>MNDPNLFVALYDFVASGDNTLSITKGEKLRVLGYNHNGEWCEAQTKNGQGWVPSNYITPVNS[2x];>APTMPP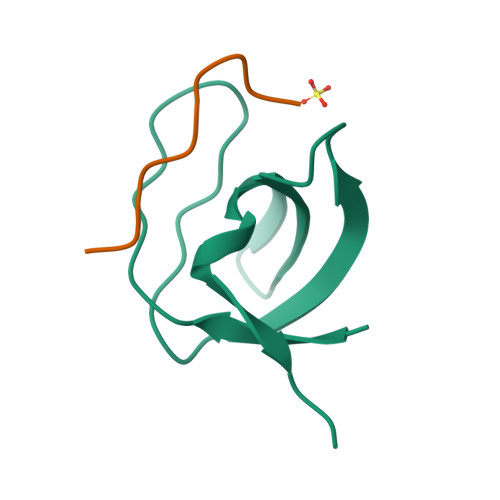PLPP[2x]>[2x]MRPLRPRAALLALLASLLAAPPVAPAEAPHLVQVDAARALWPLRRFWRSTGFCPPLPHSQADPYVLSWDQQLNLAYVGAVPHRGIKQVRTHWLLELVTTRGSTGQGLSYNF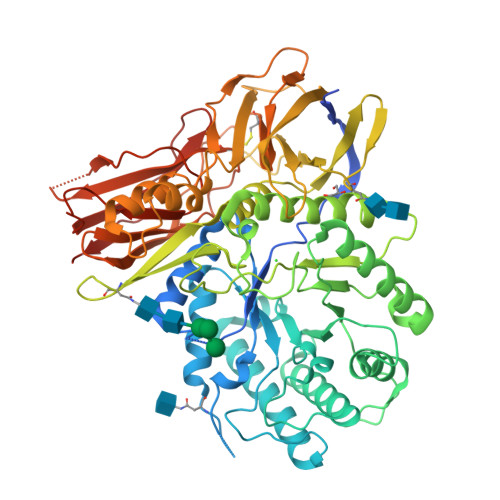THLDGYLDLLRENQLLPGFELMGSASGHFTDFEDKQQVFEWKDLVSSLARRYIGRYGLAHVSKWNFETWNEPDHHDFDNVSMTMQGFLNYYDACSEGLRAASPALRLGGPGDSFHTPPRSPLSWGLLRHCHDGTNFFTGEAGVRLDYISLHRKGARSSISILEQEKVVAQQIRQLFPKFADTPIYNDEADPLVGWSLPQPWRADVTYAAMVVKVIAQHQNLLLANTTSAFPYALLSNDNAFLSYHPHPFAQRTLTARFQVNNTRPPHVQLLRKPVLTAMGLLALLDEEQLWAEVSQAGTVLDSNHTVGVLASAHRPQGPADAWRAAVLIYASDDTRAHPNRSVAVTLRLRGVPPGPGLVYVTRYLDNGLCSPDGEWRRLGRPVFPTAEQFRRMRAAEDPVAAAPRPLPAGGRLTLRPALRLPSLLLVHVCARPEKPPGQVTRLRALPLTQGQLVLVWSDEHVGSKCLWTYEIQFSQDGKAYTPVSRKPSTFNLFVFSPDTGAVSGSYRVRALDYWARPGPFSDPVPYLEVPVPRGPPSPGNP> MSEVEDTLNRIKTHKTVLGYL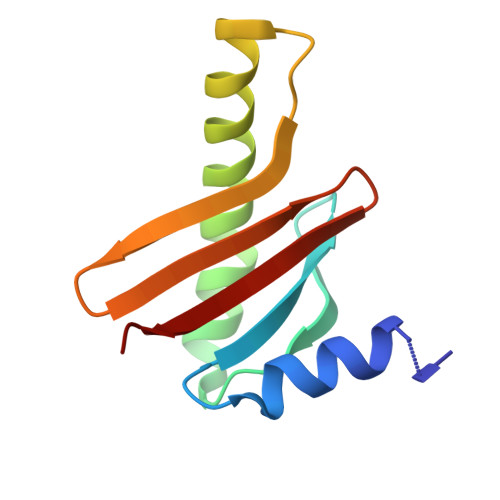IVNSEGGVVRGAFKDEEESKNIANSIPLLTKKARSVVRDLDPTNDLVFLRIQTKLNEIMVAPDDEFSLIVIQTKG Superoxide dismutases and reductases are deployed almost ubiquitously throughout nature to prevent damage to biological molecules by superoxide. They employ redox-active metal cofactors to catalyze the production of molecular oxygen and hydrogen peroxide from superoxide. Crystal structures of a Bacteroidetes bacterium CuZnSOD portray both prokaryotic and eukaryotic characteristics and propose a mechanism for self-catalyzed disulfide maturation. The Group 3 CuZnSODs described here and exemplified by BbCuZnSOD represent an evolutionary intermediary between E-class and P-class enzymes with high eukaryotic sequence identity and E-class homodimerization but P-class functional loops and disulfide configuration.

To investigate, representative Group 2 and 3a enzymes RbCuZnSOD (OUV78940) and BbCuZnSOD (OFX46851) were purified recombinantly from E. coli. BbCuZnSOD has a typical eight stranded, anti-parallel, Greek-key β-barrel core structure with two long loops incorporating conserved metal-binding ligands and coordination geometry. Comparison of BbCuZnSOD monomers with human SOD1, PhCuZnSOD and E. coli CuZnSOD monomers gives mean all-atom RMSD of 1.83 Å, 2.59 Å, and 4.22 Å, respectively. The BbCuZnSOD E-class dimer interface area is 747 Å2 comprising N-terminus, C-terminus, and disulfide subloop regions with a PISA score of 1.0 as opposed to 0.2 and 0.3 for human and bovine SOD1, respectively. Strong hydrogen bonding is facilitated by conservation of Gly150 allowing close contact between opposing Gly51 and Ile151. In addition, each Tyr14 forms two back-bone hydrogen bonds with disulfide bonding Cys146; β-barrel interactions that are conserved in human SOD1. Immediately adjacent to Tyr14 at the loop I N-terminus, Pro15 replaces a glycine which is conserved in 80.5% of eukaryotic CuZnSODs (Gly10, human SOD1). As a result, loop I adopts a conformation shifted toward the disulfide subloop.

>QVEGKTQKAVCVIYPTQDYKVTGVITFTKSDDGVKVVADLNGLSPGKHGFHIHECGDCSASDGTSAGGHFNPEEKSHGAPMDMSRHIGDLGNITADENGKAHLEYIDKMIVFEGEHSIIGRSMIVHKNEDDLKTQPTGNAGARVACGVIGIGK[4x]> MAEGKMMSDFLPFSRPAMGAEELAAVKTVLDSGWITTGPKNQELEAAFCRLTGNQYAVAVSSATAGMHIALMALGIGEGDEVITPSMTWVSTLNMIVLLGANPVMVDVDRDTLMVTPEHIEAAITPQTKAIIPVHYAGAPADLDAIYALGERYGIPVIEDAAHATGTSYKGRHIGARGTAIFSFHAIKNITCAEGGIVVTDNPQFADKLRSLKFHGLG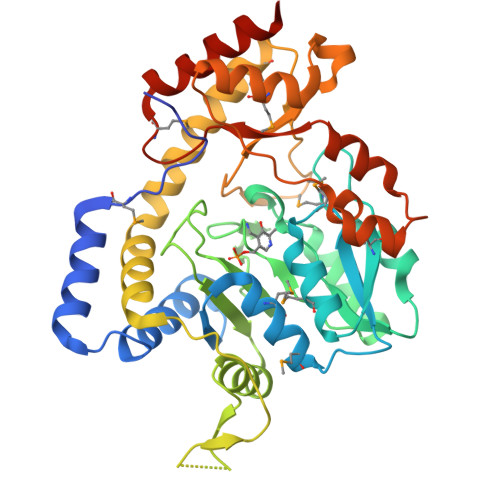VDAWDRQSGGRAPQAEVLAPGYKYNLPDLNAAIALAQLQKLDALNARRAAIAAQYHQAMADLPFQPLSLPSWEHIHAWHLFIIRVDEARCGITRDALMASLKTKGIGTGLHFRAAHTQKYYRERFPTLTLPDTEWNSERICSLPLFPDMTESDFDRVITALHQIAGQGSHHHHHH>[3x]MFVKETNRAKSPTRQSPGAAGYDLYSAYDYTIPPGERQLIKTDISMSMPKFCYGRIAPRSGLSLKGIDIGGGVIDEDYRGNIGVILINNGKCTF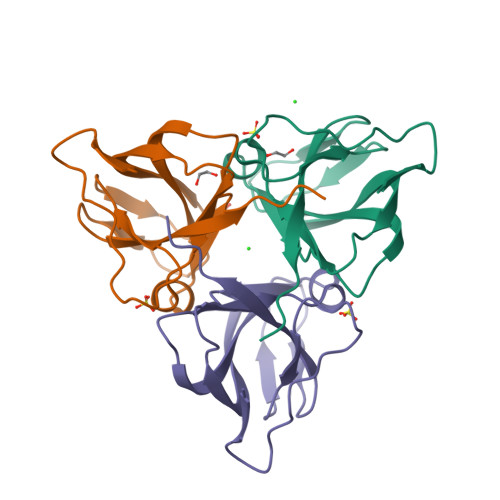NVNTGDRIAQLIYQRIYYPELEEVQSLDSTNRGDQGFGSTGLR> VDSSHLPLVKGADEEQVFHFYWLDAYEDQYNQPGVVFLFGKVWIESAETHVSCCVMVKNIERTLYFLPREMKIDLNTGKETGTPISMKDVYEEFDEKIATKYKIMKFKSKPVEKNYAFEIPDVPEKSEYLEVKYSAEMPQLPQDLKGETFSHVFGTNTSSLELFLMNRKIKGPCWLEVKSPQLLNQPVSWCKVEAMALKPDLVNVIKDVSPPPLVVMAFSMKTMQNAKNHQNEIIAMAALVHHSFALDKAAPKPPFQSHFCVVSKPKDCIFPYAFKEVIEKKNVKVEVAATERTLLGFFLAKVHKIDPDIIVGHNIYGFELEVLLQRINVCKAPHWSKIGRLKRSNMPKLGGRSGFGERNATCGRMICDVEISAKELIRCKSYHLSELVQQILKTERVVIPMENIQNMYSESSQLLYLLEHTWK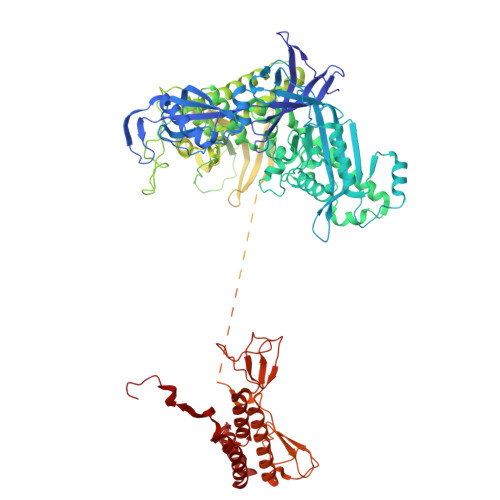DAKFILQIMCELNVLPLALQITNIAGNIMSRTLMGGRSERNEFLLLHAFYENNYIVPDKQIFRKPQQKLGDEDEEIDGDTNKYKKGRKKAAYAGGLVLDPKVGFYDKFILLLDFNSLYPSIIQEFNICFTTVQRVASEAQKVTEDGEQEQIPELPDPSLEMGILPREIRKLVERRKQVKQLMKQQDLNPDLILQYDIRQKALKLTANSMYGCLGFSYSRFYAKPLAALVTYKGREILMHTKEMVQKMNLEVIYGDTDSIMINTNSTNLEEVFKLGNKVKSEVNKLYKLLEIDIDGVFKSLLLLKKKKYAALVVEPTSDGNYVTKQELKGLDIVRRDWCDLAKDTGNFVIGQILSDQSRDTIVENIQKRLIEIGENVLNGSVPVSQFEINKALTKDPQDYPDKKSLPHVHVALWINSQGGRKVKAGDTVSYVICQDGSNLTASQRAYAPEQLQKQDNLTIDTQYYLAQQIHPVVARICEPIDGIDAVLIATWLGLDPTQFRVHHYHKDEENDALLGGPAQLTDEEKYRDCERFKCPCPTCGTENIYDNVFDGSGTDMEPSLYRCSNIDCKASPLTFTVQLSNKLIMDIRRFIKKYYDGWLICEEPTCRNRTRHLPLQFSRTGPLCPACMKATLQPEYSDKSLYTQLCFYRYIFDAECALEKLTTDHEKDKLKKQFFTPKVLQDYRKLKNTAEQFLSRSGYSEVNLSKLFAGCAVKS>GKISTDKYIFLTPRAYIIVHLLKVGKAKASEISENTQIPYQTVIQNIRWLLAEGYVVKEQKGEEI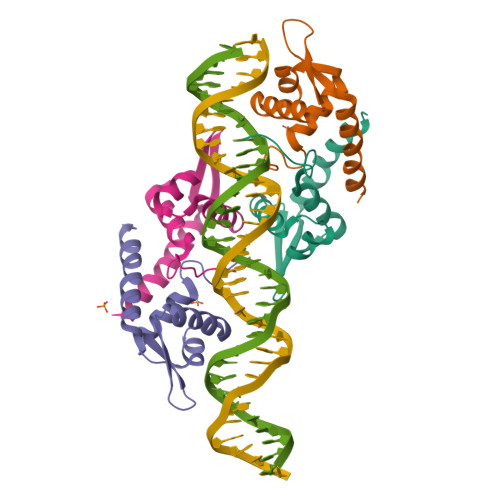YYKLTDKGKQLATAELEKIRKLVEVVQHHHHHH[6x]> MVLGKPQTDPTLEWFLSHCHIHKYPSKSTLIHQGEKAETLYYIVKGSVAVLIKDEEGKEMILSYLNQGDFIGELGLFEEGQERSAWVRAKTAC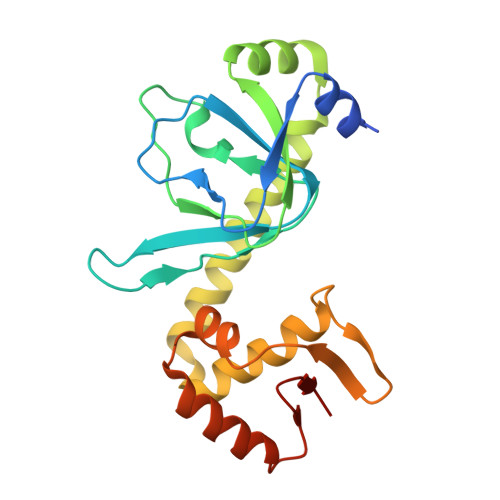EVAEISYKKFRQLIQVNPDILMRLSAQMARRLQVTSEKVGNLAFLDVTGRIAQTLLNLAKQPDAMTHPDGMQIKITRQEIGQIVGCSRETVGRILKMLEDQNLISAHGKTIVVYGTR> KNADSYAKKPHISALNAPQLDQRYKNEFTIGAAVEPYQLQNEKDVQMLKRHFNSIVAENVMKPISIQPEEGKFNFEQADRIVKFAKANGMDIRFHTLVWHSQVPQWFFLDKEGKPMVNETDPVKREQNKQLLLKRLETHIKTIVERYKDDIKYWDVVNEVVGDDGKLRNSPWYQIAGIDYIKVAFQAARKYGGDNIKLYMNDYNTEVEPKRTALYNLVKQLKEEGVPIDGIGHQSHI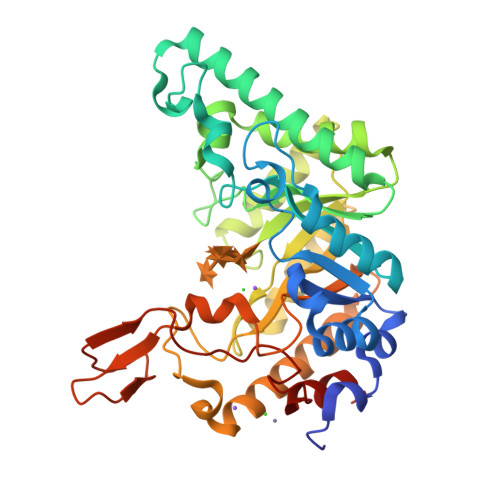QIGAPSEAEIEKTINMFAALGLDNQITELDVSMYGWPPRAYPTYDAIPKQKFLDQAARYDRLFKLYEKLSDKISNVTFWGIADNHTWLDSRADVYYDANGNVVVDPNAPYAKVEKGKGKDAPFVFGPDYKVKPAYWAIIDHK> MPVTINNFNYNDPIDNNNIIMMEPPFARGTGRYYKAFKITDRIWIIPERYTFGYKPEDFNKSSGIFNRDVCEYYDPDYLNTNDKKNIFLQTMIKLFNRIKSKPLGEKLLEMIINGIPYLGDRRVPLEEFNTNIASVTVNKLISNPGEVERKKGIFANLIIFGPGPVLNENETIDIGIQNHFASREGFGGIMQMKFCPEYVSVFNNVQENKGASIFNRRGYFSDPALILMHQLIYVLHGLYGIKVDDLPIVPNEKKFFMQSTDAIQAEELYTFGGQDPSIITPSTDKSIYDKVLQNFRGIVDRLNKVLVCISDPNININIYKNKFKDKYKFVEDSEGKYSIDVESFDKLYKSLMFGFTETNIAENYKIKTRASYFSDSLPPVKIKNLLDNEIYTIEEGFNISDKDMEKEYRGQNKAINKQAYEEISKEHLAVYKIQMCKSVKAPGICIDVDNEDLFFIADKNSFSDDLSKNERIEYNTQSNYIENDFPINELILDTDLISKIELPSENTESLTDFNVDVPVYEKQPAIKKIFTDENTIFQYLYSQTFPLDIRDISLTSSFDDALLFSNKVYSFFSMDYIKTANKVVEAGLFAGWVKQIVNDFVIEANKSNTMDKIADISLIVPYIGLALNVGNETAKGNFENAFEIAGASILLEFIPELLIPVVGAFLLESYIDNKNKIIKTIDNALTKRNEKWSDMYGLIVAQWLSTVNTQFYTIKEGMYKALNYQAQALEEIIKYRYNIYSEKEKSNINIDFNDINSKLNEGINQAIDNINNFINGCSVSYLMKKMIPLAVEKLLDFDNTLKKNLLNYIDENKLYLIGSAEYEKSKVNKYLKTIMPFDLSIYTNDTILIEMFNKYNSEILNNIILNLRYKDNNLIDLSGYGAKVEVYDGVELNDKNQFKLTSSANSKIRVTQNQNIIFNSVFLDFSVSFWIRIPKYKNDGIQNYIHNEYTIINCMKNNSGWK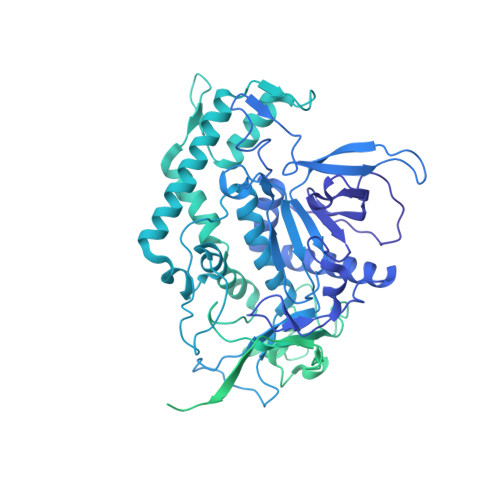ISIRGNRIIWTLIDINGKTKSVFFEYNIREDISEYINRWFFVTITNNLNNAKIYINGKLESNTDIKDIREVIANGEIIFKLDGDIDRTQFIWMKYFSIFNTELSQSNIEERYKIQSYSEYLKDFWGNPLMYNKEYYMFNAGNKNSYIKLKKDSPVGEILTRSKYNQNSKYINYRDLYIGEKFIIRRKSNSQSINDDIVRKEDYIYLDFFNLNQEWRVYTYKYFKKEEMKLFLAPIYDSDEFYNTIQIKEYDEQPTYSCQLLFKKDEESTDEIGLIGIHRFYESGIVFEEYKDYFCISKWYLKEVKRKPYNLKLGCNWQFIPKDEGWTE> TDKAYVAPEKFSSKVLTWLGKM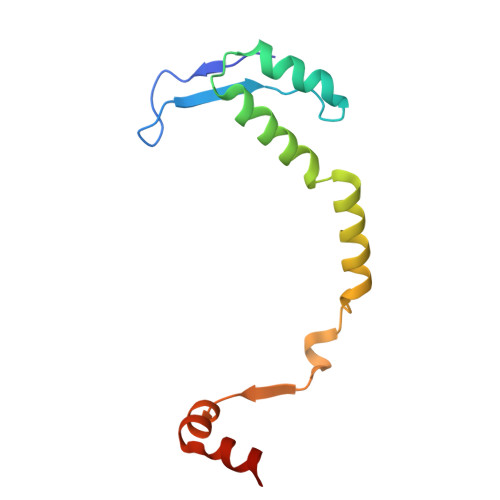PLFKNTEVVQKHTENIRVQDQKILQTFLHALTEKYGETAVNDALLMSRINMNKPLTQRLAVQITECVKAADEGFINLIKSKDN> ESCHPRLSLHRPALEDLLLGSEANLTCTLTGLRDASG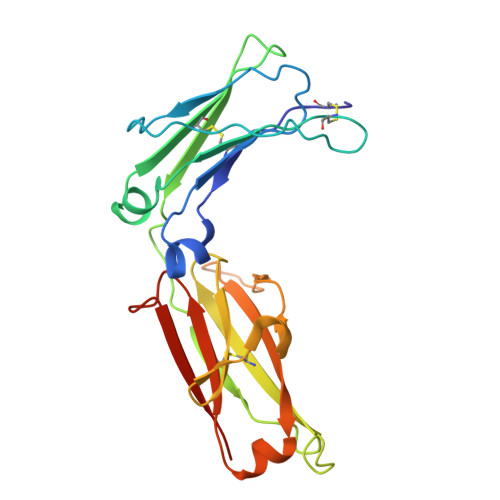VTFTWTPSSGKSAVQGPPERDLCGCYSVSSVLPGCAEPWNHGKTFTCTAAYPESKTPLTATLSKSGNTFRPEVHLLPPPSEELALNELVTLTCLARGFSPKDVLVRWLQGSQELPREKYLTWASRQEPSQGTTTFAVTSILRVAAEDWKKGDTFSCMVGHEALPLAFTQKTIDRLAGKP> MLVHYGKLSDMPTVVDVNTTMGTDVPEDL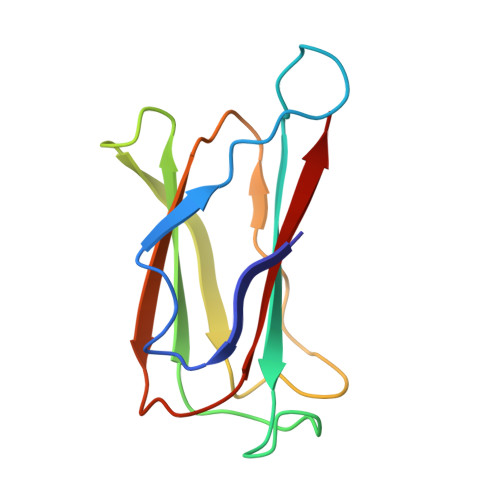LEIYVGCYAADGKTPAAGTGVLTFHGSWNGVHKRLIGTVDLAAAGEVIAYNPPLMFGGCKKLFVSYTGVGTQIVDVYVHRGE> ARPTVIRWSE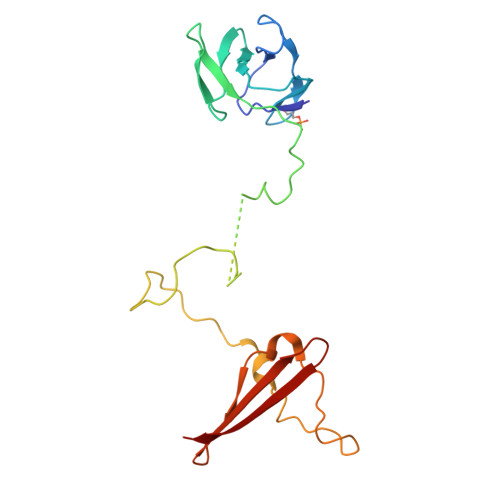GGKEVFISGSFNNWSTKIPLIKSHNDFVAILDLPEGEHQYKFFVDGQWVHDPSEPVVTSQLGTINNLIHVKKSDFEVFDALKLDSMESSETSCRDLSSSPPGPYGQEMYAFRSEERFKSPPILPPHLLQVILNKDTNISCDPALLPEPNHVMLNHLYALSIKDSVMVLSATHRYKKKYVTTLLYKPI>MASSLRAAISKIKRDDVGQQVCPNYVMLRSSVTTKVVRNVVEYQIRTGGFFSCLAMLRPLQYAKRERLLGQRNLERISTRDILQTRDLHSLCMPTPDAPMSNHQASTMRELICSYFKVDHADGLKYIPMDERYSPSSLARLFTMGMAGLHITTEPSYKRVPIMHLAADLDCMTLALPYMITLDGDTVVPVAPTLSAEQLLDDGLKGLACMDISYGCEVDANSRPAGDQSMDSSRCINELYCEETA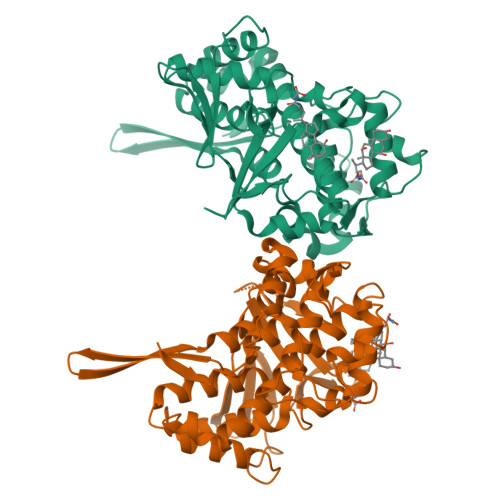EAICVLKTCLVLNCMQFKLEMDDLAHNAAELDKIQMMIPFSERVFRMASSFATIDAQCFRFCVMMKDKNLKIDMRETTRLWTRSASDDSVATSSLSISLDRGRWVAADASDARLLVFPIRV[2x]> GSMPPQLHNGLDFSAKVIQGSLDSLPQEVRKFVEGNAQLCQPEYIHICDGSEEEYGRLLAHMQEEGVIRKLKKYDNCWLALTDPRDVARIESKTVIITQEQRDTVPIPKSGQSQLGRWMSEEDFEKAFNARFPGCMKGRTMYVIPFSMGPLGSPLAKIGIELTDSPYVVASMRIMTRMGTSVLEALGDGEFIKCLHSVGCPLPLKKPLVNNWACNPELTLIAHLPDRREIISFGSGYGGNSLLGKKCFALRIASRLAKEEGWLAEHMLILGITNPEGKKKYLAAAFPSACGKTNLAMMNPTLPGWKVECVGDDIAWMKFDAQGNLRAINPENGFFGVAPGTSVKTNPNAIKT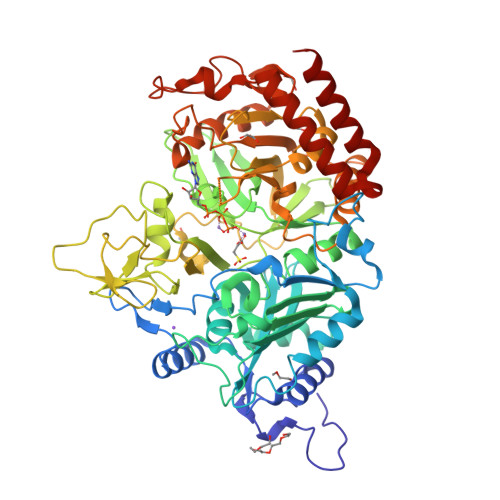IQKNTIFTNVAETSDGGVYWEGIDEPLAPGVTITSWKNKEWRPQDEEPCAHPNSRFCTPASQCPIIDPAWESPEGVPIEGIIFGGRRPAGVPLVYEALSWQHGVFVGAAMRSEATAGAEHKGKVIMHDPFAMRPFFGYNFGKYLAHWLSMAHRPAAKLPKIFHVNWFRKDKNGKFLWPGFGENSRVLEWMFGRIEGEDSAKLTPIGYVPKEDALNLKGLGDVNVEELFGISKEFWEKEVEEIDKYLEDQVNADLPYEIERELRALKQRISQM> MTPEAIIEDRRFQETLDKIRKEEGYDFAAIAFYESNKPSSPIKWHYVSGNKNNRFKLIILRKGRGLAGTVMKTGKRMVIANVGLALGPEEKIDYPILLSESLTAVLAVPLWYKNQVYGVLLFGQRDGR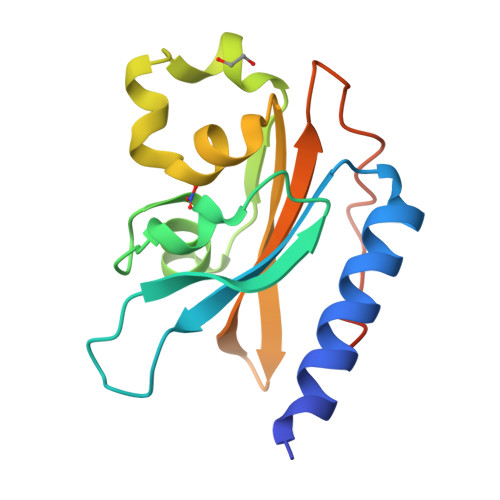PLPKIFDNDDIQRKFGIFNDDK> MLKRIKIVTSLLLVLAVFGLLQLTSGGLFFNALKNDKENFTVLQTIRQQQSTLNG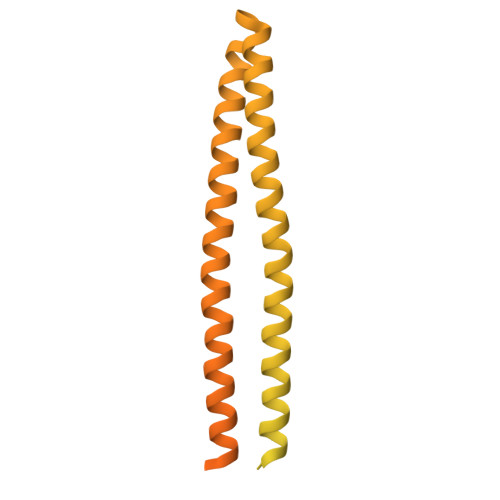SWVALLQTRNTLNRAGIRYMMDQNNIGSGSTVAELMESASISLKQAEKNWADYEALPRDPRQSTAAAAEIKRNYDIYHNALAELIQLLGAGKINEFFDQPTQGYQDGFEKQYVAYMEQNDRLHDIAVSDNNASYSQAMWILVGVMIVVLAVIFAVWFGIKASLVAPMNRLIDSIRHIAGGDLVKPIEVDGSNEMGQLAESLRHMQGELMRTVGDVRNGANAIYSGASEIATGNNDLSSRTEQQAASLEETAASMEQLTATVKQNAENARQASHLALSASETAQRGGKVVDNVVQTMRDISTSSQKIADIISVIDGIAFQTNILALNAAVEAARAGEQGRGFAVVAGEVRNLAQRSAQAAREIKSLIEDSVGKVDVGSTLVESAGETMAEIVSAVTRVTDIMGEIASASDEQSRGIDQVGLAVAEMDRVTQQNAALVEESAAAAAALEEQASRLTEAVAVFRIQQQQRETSAVVKTVTPAAPRKMAVADSEENWETF>AVKVKVP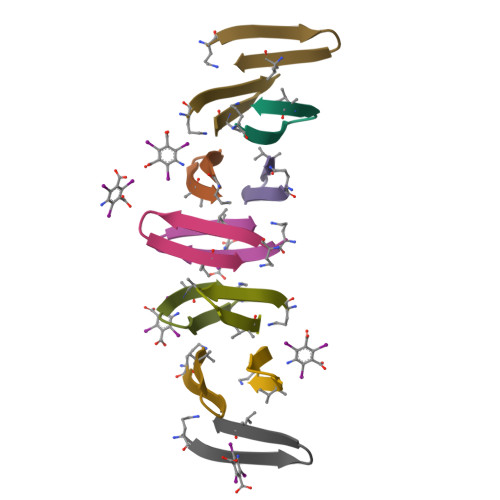PTKXKV[12x]> AMGSPIQVIENDRASRGGQVYATNTRGQIPPLVTTDCMIQDQGNASPRFIRCTTYCFPCTSDMAKQAQIPLAAVIKPFATIPSNESPLYLVNHGESGPVRCNRCKAYMCPFMQFIEGGRRYQCGFCNCVND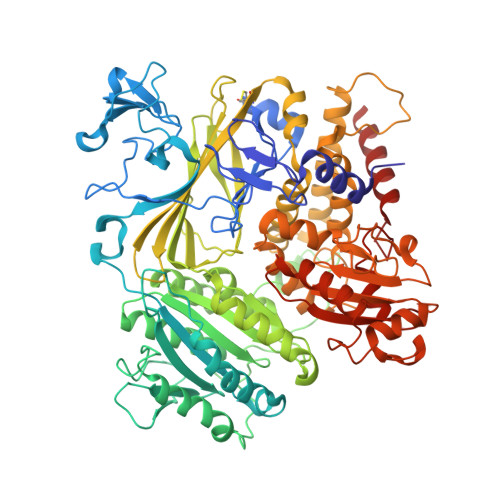VPPFYFQHLDHIGRRLDHYEKPELSLGSYEYVATLDYCRKSKPPNPPAFIFMIDVSYSNIKNGLVKLICEELKTMLEKIPKEEQEETSAIRVGFITYNKVLHFFNVKSNLAQPQMMVVTDVGEVFVPLLDGFLVNYQESQSVIHNLLDQIPDMFADSNENETVFAPVIQAGMEALKAADCPGKLFIFHSSLPTAEAPGKLKNRDDKKLVNTDKEKILFQPQTNVYDSLAKDCVAHGCSVTLFLFPSQYVDVASLGLVPQLTGGTLYKYNNFQMHLDRQQFLNDLRNDIEKKIGFDAIMRVRTSTGFRATDFFGGILMNNTTDVEMAAIDCDKAVTVEFKHDDKLSEDSGALIQCAVLYTTISGQRRLRIHNLGLNCSSQLADLYKSCETDALINFFAKSAFKAVLHQPLKVIREILVNQTAHMLACYRKNCASPSAASQLILPDSMKVLPVYMNCLLKNCVLLSRPEISTDERAYQRQLVMTMGVADSQLFFYPQLLPIHTLDVKSTMLPAAVRCSESRLSEEGIFLLANGLHMFLWLGVSSPPELIQGIFNVPSFAHINTDMTLLPEVGNPYSQQLRMIMGIIQQKRPYSMKLTIVKQREQPEMVFRQFLVEDKGLYGGSSYVDFLCCVHKEICQLLN> AGTMVGNREEKILNREIGFAIGMPVCEFDMVKDPEVQDFRRNILNVCKEAVDLRDLNSPHSRAMYVYPPNVESSPELPKHIYNKLDKGQIIVVIWVIVSPNNDKQKYTLKINHDCVPEQVIAEAIRKKTRSMLLSSEQLKLCVLEYQGKYILKVCGCDEYFLEKYPLSQYKYIRSCIMLGRMPNLMLMAKESLYSQLPMDCFTMPSYSRRISTATPYMNGETSTKSLWVINSALRIKILCATYVNVNIRDIDKIYVRTGIYHGGEPLCDNVNTQRVPCSNPRWNEWLNYDIYIPDLPRAARLCLSICSVKGRKGAKEEHCPLAWGNINLFDYTDTLVSGKMALNLWPVPHGLEDLLNPIGVTGSNPNKETPCLELEFDWFSSVVKFPDMSVIEEHANWSVSREAGFSYSHAGLSNRLARDNELRENDKEQLKAISTRDPLSEITEQEKDFLWSHRHYCVTIPEILPKLLLSVKWNSRDEVAQMYCLVKDWPPIKPEQAMELLDCNYPDPMVRGFAVRCLEKYLTDDKLSQYLIQLVQVLKYEQYLDNLLVRFLLKKALTNQRIGHFFFWHLKSEMHNKTVSQRFGLLLESYCRACGMYLKHLNRQVEAMEKLINLTDILKQEKKDETQKVQMKFLVEQMRRPDFMDALQGFLS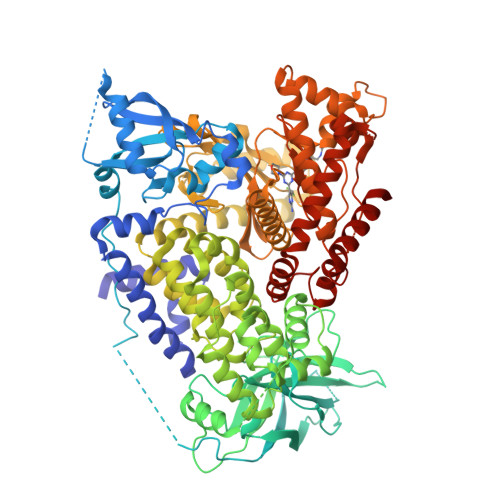PLNPAHQLGNLRLEECRIMSSAKRPLWLNWENPDIMSELLFQNNEIIFKNGDDLRQDMLTLQIIRIMENIWQNQGLDLRMLPYGCLSIGDCVGLIEVVRNSHTIMQIQCKGGLKGALQFNSHTLHQWLKDKNKGEIYDAAIDLFTRSCAGYCVATFILGIGDRHNSNIMVKDDGQLFHIDFGHFLDHKKKKFGYKRERVPFVLTQDFLIVISKGAQECTKTREFERFQEMCYKAYLAIRQHANLFINLFSMMLGSGMPELQSFDDIAYIRKTLALDKTEQEALEYFMKQMNDAHH> MMFGKKKNNGGSSTARYSAGNKYNTLSNNYALSAQQLLNASKIDDIDSMMGFERYVPPQYNGRFDAKDIDQIPGRVGWLTNMHATLVSQETLSSGSNGGGNSNDGERVTTNQGISGVDFYFLDEEGGSFKSTVVYDPYFFIACNDESRVNDVEELVKKYLESCLKSLQIIRKEDLTMDNHLLGLQKTLIKLSFVNSNQLFEARKLLRPILQDNANNNVQRNIYNV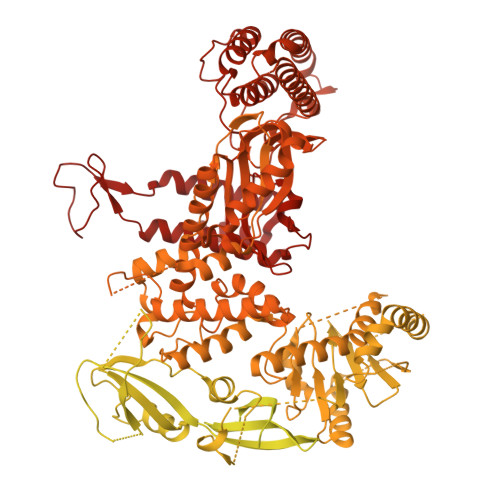AANGSEKVDAKHLIEDIREYDVPYHVRVSIDKDIRVGKWYKVTQQGFIEDTRKIAFADPVVMAFAIATTKPPLKFPDSAVDQIMMISYMIDGEGFLITNREIISEDIEDFEYTPKPEYPGFFTIFNENDEVALLQRFFEHIRDVRPTVISTFNGDFFDWPFIHNRSKIHGLDMFDEIGFAPDAEGEYKSSYCSHMDCFRWVKRDSYLPQGSQGLKAVTQSKLGYNPIELDPELMTPYAFEKPQHLSEYSVSDAVATYYLYMKYVHPFIFSLCTIIPLNPDETLRKGTGTLCEMLLMVQAYQHNILLPNKHTDPIERFYDGHLLESETYVGGHVESLEAGVFRSDLKNEFKIDPSAIDELLQELPEALKFSVEVENKSSVDKVTNFEEIKNQITQKLLELKENNIRNELPLIYHVDVASMYPNIMTTNRLQPDSIKAERDCASCDFNRPGKTCARKLKWAWRGEFFPSKMDEYNMIKRALQNETFPNKNKFSKKKVLTFDELSYADQVIHIKKRLTEYSRKVYHRVKVSEIVEREAIVCQRENPFYVDTVKSFRDRRYEFKGLAKTWKGNLSKIDPSDKHARDEAKKMIVLYDSLQLAHKVILNSFYGYVMRKGSRWYSMEMAGITCLTGATIIQMARALVERVGRPLELDTDGIWCILPKSFPETYFFTLENGKKLYLSYPCSMLNYRVHQKFTNHQYQELKDPLNYIYETHSENTIFFEVDGPYKAMILPSSKEEGKGIKKRYAVFNEDGSLAELKGFELKRRGELQLIKNFQSDIFKVFLEGDTLEGCYSAVASVCNRWLDVLDSHGLMLEDEDLVSLICENRSMSKTLKEYEGQKSTSITTARRLGDFLGEDMVKDKGLQCKYIISSKPFNAPVTERAIPVAIFSADIPIKRSFLRRWTLDPSLEDLDIRTIIDWGYYRERLGSAIQKIITIPAALQGVSNPVPRVEHPDWLKRKIATKEDKFKQTSLTKFFSKTKNVPTMGKIKDIEDLFEPTVEEDNAKIKIARTTKKKAVSKRKRNQLTNEEDPLVLPSEIPSMDEDYVGWLNYQKIKWKIQARDRKRRDQLFGNTNSSRERSALGSMIRKQAESYANSTWEVLQYKDSGEPGVLEVFVTINGKVQNITFHIPKTIYMKFKSQTMPLQKIKNCLIEKSSASLPNNPKTSNPAGGQLFKITLPESVFLEEKENCTSIFNDENVLGVFEGTITPHQRAIMDLGASVTFRSKAMGALGKGIQQGFEMKDLSMAENERYLSGFSMDIGYLLHFPTSIGYEFFSLFKSWGDTITILVLKPSNQAQEINASSLGQIYKQMFEKKKGKIETYSYLVDIKEDINFEFVYFTDISKLYRRLSQETTKLKEERGLQFLLLLQSPFITKLLGTIRLLNQMPIVKLSLNEVLLPQLNWQPTLLKKLVNHVLSSGSWISHLIKLSQYSNIPICNLRLDSMDYIIDVLYARKLKKENIVLWWNEKAPLPDHGGIQNDFDLNTSWIMNDSEFPKINNSGVYDNVVLDVGVDNLTVNTILTSALINDAEGSDLVNNNMGIDDKDAVINSPSEFVHDAFSNDALNVLRGMLKEWWDEALKENSTADLLVNSLASWVQNPNAKLFDGLLRYHVHNLTKKALLQLVNEFSALGSTIVYADRNQILIKTNKYSPENCYAYSQYMMKAVRTNPMFSYLDLNIKRYWDLLIWMDKFNFSGLACIEIEEKENQDYTAVSQWQLKKFLSPIYQPEFEDWMMIILDSMLKTKQSYLKLNSGTQRPTQIVNVKKQDKEDSVENSLNGFSHLFSKPLMKRVKKLFKNQQEFILDPQYEADYVIPVLPGSHLNVKNPLLELVKSLCHVMLLSKSTILEIRTLRKELLKIFELREFAKVAEFKDPSLSLVVPDFLCEYCFFISDIDFCKAAPESIFSCVRCHKAFNQVLLQEHLIQKLRSDIESYLIQDLRCSRCHKVKRDYMSAHCPCAGAWEGTLPRESIVQKLNVFKQVAKYYGFDILLSCIADLTI>[2x]GSMR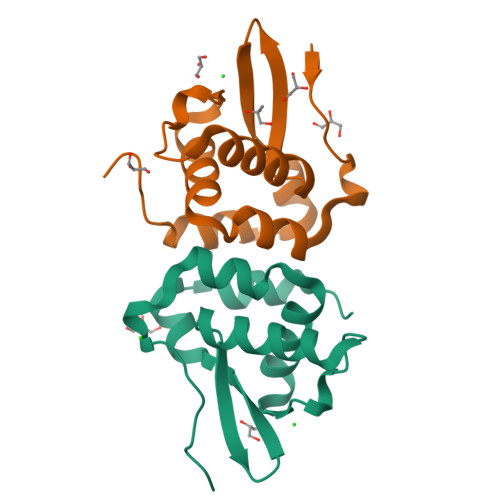FLYHPDRKDISLPGVLYALGDPARLEIVRLLASKGEQCCAEFDFAIAKSTMSNHFKILRESGVVLTRKEGTQHINRLRREDLETLFPGLLDAVLRSAQPLLTCQQSAIVK2-[(2~{S})-1-[2-[methyl-(1-methylpiperidin-4-yl)amino]thieno[3,2-d]pyrimidin-4-yl]-2,3-dihydropyrrol-2-yl]ethanenitrile | C19 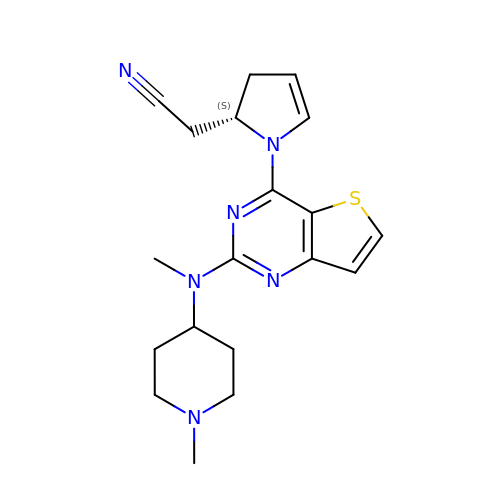H24 N6 S | ZMXVLDNFPUUWQK-HNNXBMFYSA-N>MAEFRIAQDVVARENDRRASALKEDYEALGANLARRGVDIEAVTAKVEKFFVAVPSWGVGTGGTRFARFPGTGEPRGIFDKLDDCAVIQQLTRATPNVSLHIPWDKADPKELKAR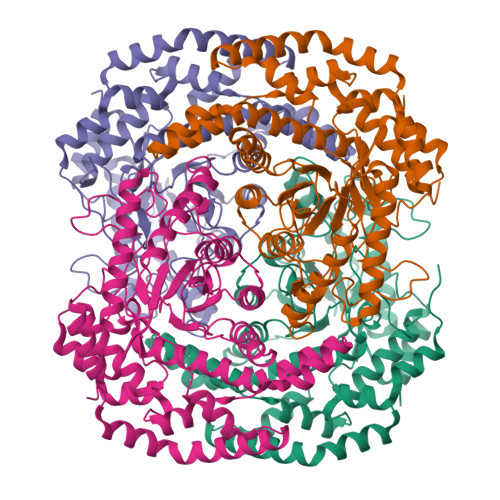GDALGLGFDAMNSNTFSDAPGQAHSYKYGSLSHTNAATRAQAVEHNLECIEIGKAIGSKALTVWIGDGSNFPGQSNFTRAFERYLSAMAEIYKGLPDDWKLFSEHKMYEPAFYSTVVQDWGTNYLIAQTLGPKAQCLVDLGHHAPNTNIEMIVARLIQFGKLGGFHFNDSKYGDDDLDAGAIEPYRLFLVFNELVDAEARGVKGFHPAHMIDQAHNVTDPIESLINSANEIRRAYAQALLVDRAALSGYQEDNDALMATETLKRAYRTDVEPILAEARRRTGGAVDPVATYRASGYRARVAAERPASVAGGGGIIGSHHHHHH[4x]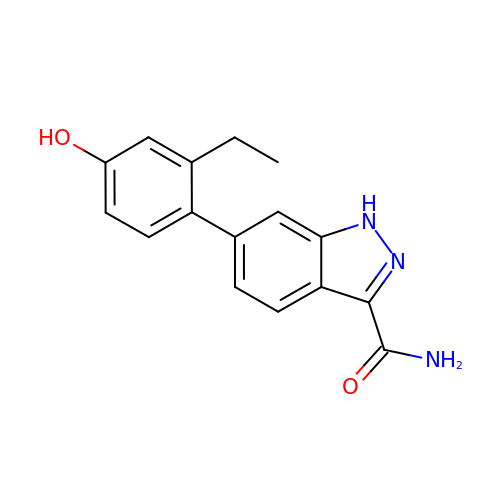6-(2-ethyl-4-hydroxyphenyl)-1H-indazole-3-carboxamide | C16 H15 N3 O2 | MSKMVINDTCVTEK-UHFFFAOYSA-N methyl N-(carboxymethyl)-N-(3-phenylpropanoyl)glycyl-D-histidinate 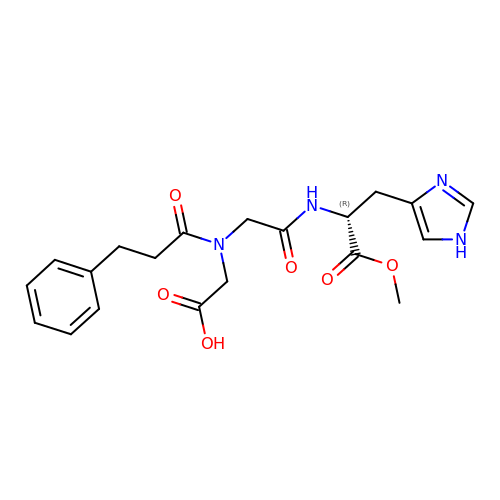| C20 H24 N4 O6 | FTBNIEVYMZAOPN-MRXNPFEDSA-N> VIHVTKEVKEVATLSCGHNVSVEELAQTRIYWQKEKK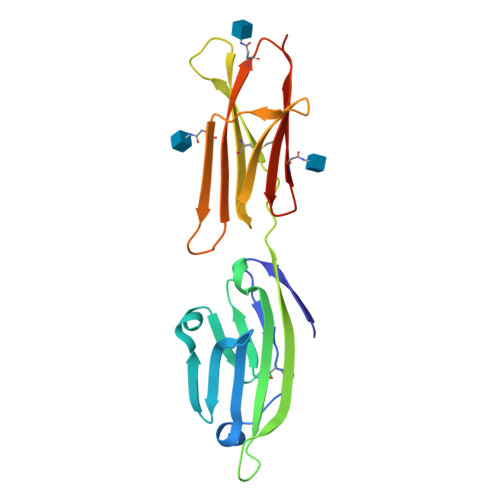MVLTMMSGDMNIWPEYKNRTIFDITNNLSIVILALRPSDEGTYECVVLKYEKDAFKREHLAEVTLSVKADFPTPSISDFEIPTSNIRRIICSTSGGFPEPHLSWLENGEELNAINTTVSQDPETELYAVSSKLDFNMTTNHSFMCLIKYGHLRVNQTFNWNTAK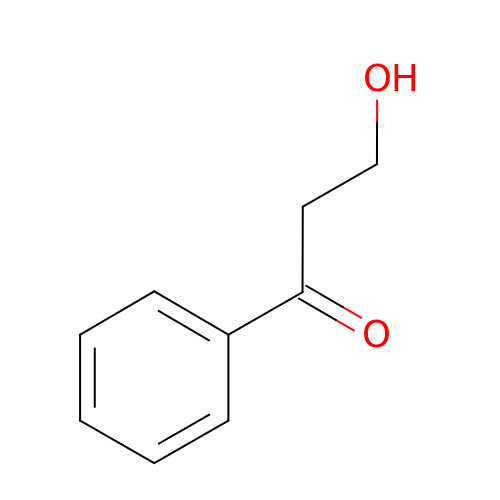3-hydroxy-1-phenylpropan-1-one | C9 H10 O2 | PQCFUZMQHVIOSM-UHFFFAOYSA-N>[2x]MERINFIFGIHNHQPLGNFGWVFEEAYNRSYRPFMEILEEFPEMKVNVHFSGPLLEWIEENKPDYLDLLRSLIKRGQLEIVVAGFYEPVLAAIPKEDRLVQIEMLKDYARKLGYDAKGVWLTERVWQPELVKSLREAGIEYVVVDDYHFMSAGLSKEELFWPYYTEDGGEVITVFPIDEKLRYLIPFRP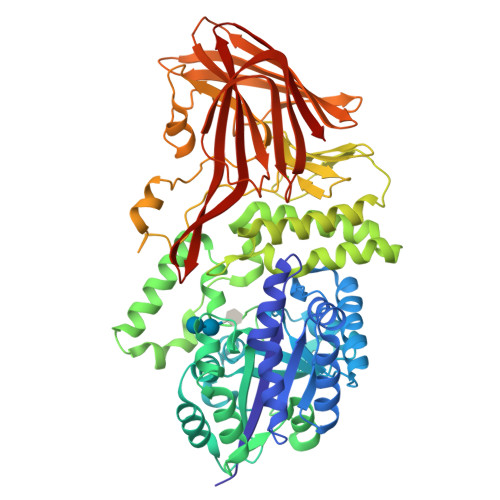VKKTIEYLESLTSDDPSKVAVFHDDGEKFGVWPGTYEWVYEKGWLREFFDAITSNEKINLMTYSEYLSKFTPRGLVYLPIASYFEMSEWSLPAKQAKLFVEFVEQLKEEGKFEKYRVFVRGGIWKNFFFKYPESNFMHKRMLMVSKAVRDNPEARKYILKAQCNDAYWHGVFGGIYLPHLRRTVWENIIKAQRYLKPENKILDVDFDGRAEIMVENDGFIATIKPHYGGSIFELSSKRKAVNYNDVLPRRWEHYHEVPEATKPEKESEEGIASIHELGKQIPEEIRRELAYDWQLRAILQDHFIKPEETLDNYRLVKYHELGDFVNQPYEYEMIENGVKLWREGGVYAEEKIPARVEKKIELTEDGFIAKYRVLLEKPYKALFGVEINLAVHSVMEKPEEFEAKEFEVNDPYGIGKVRIELDKAAKVWKFPIKTLSQSEAGWDFIQQGVSYTMLFPIEKELEFTVRFREL>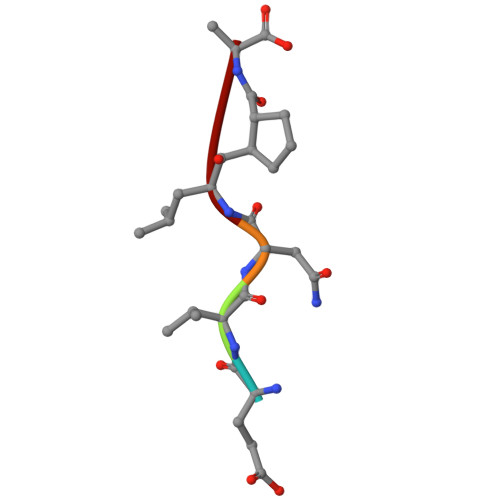 EVNXA>[2x]MGHHHHHHSGENLYFQGTIRSYKNLNLVRANIETESRQFIENKNYSIQSIGPMPGSRAGLRVVFTRPGVNLATVDIFYNGDGSTTIQYLTGANRSLGQELADHLFETINPAEFEQVNMVLQGFVETSVLPVLELSADESHIEFREHSRNAHTVVWKIISTSYQDELTVSLHI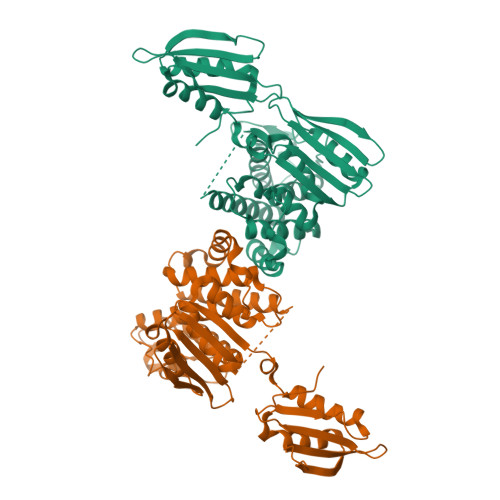TTGKLQIQGRPLSCYRVFTFNLAALLDLQGLEKVLIRQEDGKANIVQQEVARTYLQTVMADAYPHLHVTAEKLLVSGLCVKLAAPDLPDYCMLLYPELRTIEGVLKSKMSGLGMPVQQPAGFGTYFDKPAAHYILKPQFAATLRPEQINIISTAYTFFNVEAHSLFHMETVVDASRMISDMARLMGKATRAWGIIKDLYIV> SRNVPFPYAETDVADLQARMTAGELDSTTLTQAYLQRIAALDRTGPRLRAVIELNPDALKEAAERDRERRDGRLRGPLHGIPLLLKDNINAAPMATSAGSLALQGFRPDDAYLVRRLRDAGAVVLGKTNLSEWANFRGNDSISGWSARGGQTRNPYRISHSPCGSSSGSAVAVAANLASVAIGTETDGSIVCPAAINGVVGLKPTVGLVSRDGIIPISFSQDTAGPMARSVADAAAVLTAIAGRDDADPATATMPGRAVYDYTARLDPQGLRGKRIGLLQTPLLKYRGMPPLIEQAATELRRAGAVVVPVELPNQGAWAEAERTLLLYEFKAGLERYFNTHRAPLRSLADLIAFNQAHSKQELGLFGQELLVEADATAGLADPAYIRARSDARRLAGPEGIDAALAAHQLDALVAPTTGVAWPIRSEGDDFPGESYSAAAVAGYPSLTVPMGQIDGLPVGLLFMGTAWS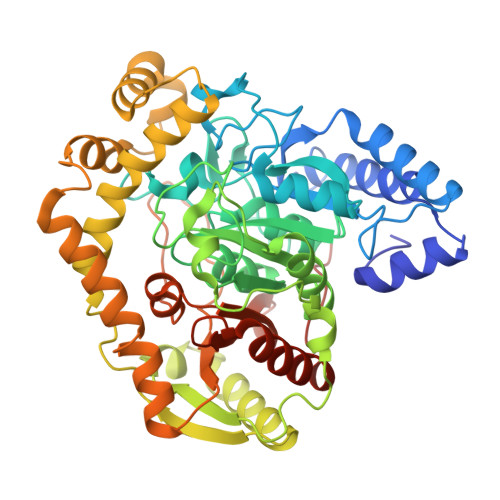EPKLIEMAYAYEQRTRARRPPHFDTDALIDAGEP>MPHFTVTKVEDPEEGAAASISQEPSLADIKARIQDSDEPDLSQNDITGEHSQLLDDGHKKARNAYLNNSNYEEGDEYFDKNLALFEEEMDTRPKVSSLLNRMANYTNLTQGAKEHEEAENITEGKKKPTKTPQMGTFMGVYLPCLQNIFGVILFLRLTWVVGTAGVLQAFAIVLICCCCTMLTAISMSAIATNGVVPAGGSYFMISRALGPEFGGAVGLCFYLGTTFAAAMYILGAIEIFLVYIVPRAAIFHSDDALKESAAMLNNMRVYGTAFLVLMVLVVFIGVRYVNKFASLFLACVIVSILAIYAGAIKSSFAPPHFPVCMLGNRTLSSRHIDVCSKTKEINNMTVPSKLWGFFCNSSQFFNATCDEYFVHNNVTSIQGIPGLASGIITENLWSNYLPKGEIIEKPSAKSSDVLGSLNHEYVLVDITTSFTLLVGIFFPSVTGIMAGSNRSGDLKDAQKSIPIGTILAILTTSFVYLSNVVLFGACIEGVVLRDKFGDAVKGNLVVGTLSWPSPWVIVIGSFFSTCGAGLQSLTGAPRLLQAIAKDNIIPFLRVFGHSKANGEPTWALLLTAAIAELGILIASLDLVAPILSMFFLMCYLFVNLACALQTLLRTPNWRPRFRYYHWALSFMGMSICLALMFISSWYYAIVAMVIAGMIYKYIEYQGAEKEWGDGIRGLSLSAARFALLRLEEGPPHTKNWRPQLLVLLKLDEDLHVKHPRLLTFASQLKAGKGLTIVGSVIVGNFLENYGEALAAEQTIKHLMEAEKVKGFCQLVVAAKLREGISHLIQSCGLGGMKHNTVVMGWPNGWRQSEDARAWKTFIGTVRVTTAAHLALLVAKNISFFPSNVEQFSEGNIDVWWIVHDGGMLMLLPFLLKQHKVWRKCSIRIFTVAQLEDNSIQMKKDLATFLYHLRIEAEVEVVEMHDSDISAYTYERDLMMEQRSQMLRHMRLSKTERDREAQLVKDRNSMLRLTSIGSDEDEETETYQEKVHMDWTKDKYMASRGQKAKSMEGFQDLLNMRPDQSNVRRMHTAVKLNEVIVNKSHEAKLVLLNMPGPPRNPEGDENYMEFLEVLTEGLERVLLVRGGGSEVITIYSA[2x]

Potassium‐coupled chloride transporters (KCCs) play crucial roles in regulating cell volume and intracellular chloride concentration. They are characteristically inhibited under isotonic conditions via phospho‐regulatory sites located within the cytoplasmic termini. Decreased inhibitory phosphorylation in response to hypotonic cell swelling stimulates transport activity, and dysfunction of this regulatory process has been associated with various human diseases. Here, we present cryo‐EM structures of human KCC3b and KCC1, revealing structural determinants for phospho‐regulation in both N‐ and C‐termini.

To understand the structural basis of phospho‐regulation in potassium‐coupled chloride transporters, we used single‐particle cryo‐electron microscopy to study the full‐length wild‐type KCC3b transporter and mutants of this transporter in which two canonical threonines (T940 and T997) and a third KCC3‐specific phosphorylation site (S45), which was shown to play a role for full activation in response to swelling (Melo et␣al, 2013), were replaced. We show that phospho‐mimetic KCC3b is arrested in an inward‐facing state in which intracellular ion access is blocked by extensive contacts with the N‐terminus. A unique feature observed in the phospho‐mimetic KCC3b‐PM structure is the presence of pronounced density for a short stretch of the otherwise unstructured N‐terminus, a domain that has not been resolved in any of the previously published CCC structures. Electrostatic surface representations of KCC3b in absence or presence of the N‐terminus illustrate that this segment is wedged between CTD and TMD and partially inserted into the inward‐open vestibule created by the helical arrangement of TM2, TM7 and the helices TM1a and TM6b of the transporter core domain. The direct contact with the ion coordinating helices TM1a and TM6b results in a visible obstruction of the ion access path from the intracellular side, suggesting that this domain arrangement could play a role in controlling transport activity. While this structure was obtained under K+‐free conditions (Fig EV2A), we see the same configuration of the N‐terminus in a lower resolution structure of KCC3b‐PM in presence of K+ (Fig EV2D). Density for N‐terminal helix (purple cartoon) is visible in the cryo‐EM maps of KCC3b‐PM in detergent environments, in both potassium‐free (A) and potassium‐saturated (D) conditions.>[2x]MAGAVGRPRRSAPRRAGKNPREEILDASAELFTHQGFATTSTHQIADAVGIRQASLYYHFPSKTEIFLTLLKSTVEPSTVLAEDLS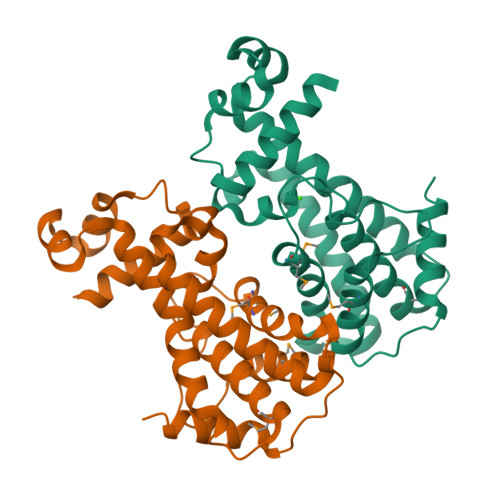ILDAGPEMRLWAIVASEVRLLLSTKWNVGRLYQLPIVGSEEFAEYHSQREALTNIFRDLATEIVGDDPRAELPFHITMSVIEMRRNDGKIPSPLSADSLPETAIMLADASLAVLGASLPADRVEKTLELIKQADAK>[2x]MNSPQNVSTKKVTVTGAAGQISYSLLWRIANGEVFGTDTPVELKLLEIPQALGGAEGVAMELLDSAFPLLRNITITADANEAFDGANAAFLVGAKPRGKGEERADLLANNGKIFGPQGKAINDNAADDIRVLVVGNPANTNALIASAAAPDVPASRFNAMMRLDHNRAISQLATKLGRGSAEFNNIVVWGNHSATQFPDITYATVGGEKVTDLVDHDWYVEEFIPRVANRGAEIIEVRGKSSAASAASSAIDHMRDWVQGTEAWSSAAIPSTGAYGIPEGIFVGLPTVSRNGEWEIVEGLEISDFQRARIDANAQELQAEREAVRDLLLEHHHHHH

The key enzymes involved in SA production were identified to be phosphoenolpyruvate (PEP) carboxykinase (PCKA) that converts PEP to oxaloacetate (OAA) while producing ATP, malate dehydrogenase (MDH) that reduces OAA to malate using NADH as a cofactor, fumarase (FUMC) that converts malate to fumarate, and fumarate reductase (FRD) that reduces fumarate to SA using menaquinol as a cofactor. Among these key enzymes, the NAD+/NADH-dependent MDH was predicted to be important for further engineering as it converts OAA to malate, which is a committed step toward SA biosynthesis. The crystal structures of MsMDH and CgMDH were determined and detailed structural comparison was carried out. The two structures, representing the mitochondrial and cytosolic MDHs, were identified to be quite different from each other with a root-mean-square deviation value of 2.77.

However, the MDHs from the major microorganisms employed for SA overproduction, such as A. succinogenes, E. coli, M. succiniciproducens, S. cerevisiae, and Y. lipolytica are clustered together with the mitochondrial MDH family, whereas the C. glutamicum MDH belongs to the cytosolic MDH family. CgMDH showed high activity at relatively acidic pH and the highest activity at pH 7.0, whereas MsMDH showed the highest activity at pH 9.0 and dramatically reduced activity at acidic pH. At pH 5.0–7.0, CgMDH exhibited significantly higher kcat compared with MsMDH, which is consistent with the results of the optimal pH study above. On the other hand, CgMDH activity was reduced only to a small degree due to relatively mild substrate inhibition as reflected by its high ki values over the entire pH range. Noticeable differences in the substrate (OAA or malate) and cofactor (NADH or NAD+) binding sites of MsMDH and CgMDH were found from the conformation of mobile loop36 and the lengths of β7-β8, α2-β2, and α7-α8 connecting loops. The β7-β8, α2-β2, and α7-α8 connecting loops include a catalytic histidine residue, the NADH-stabilizing residues, and the OAA-binding residues, respectively. Presence of a protruding Gln20 in CgMDH was also observed at the pyrophosphate moiety binding site, whereas MsMDH was found to possess Gly11 instead. One of the variants, MsMDHG11Q, showed 2.9-fold higher activity compared with MsMDH, whereas the activity of the CgMDHQ20G variant (the counterpart variant of MsMDHG11Q) was reduced compared with CgMDH. The SA production performance had significantly decreased compared with the PALK (pMS3-cgmdh) strain, indicating decreased catalytic performance of substituting Gln20 of CgMDH with glycine. Fed-batch culture of the PALK (pMS3-cgmdh) strain produced 87.23 g L−1 of SA with yield and productivity of 1.29 mol mol−1 glucose and 3.6 g L−1 h−1, respectively; the titer, yield, and productivity all significantly increased by amplifying the cgmdh gene.>RTKIVVKVHMPCDKSRAKAVALAASVNGVDVVEITGEDKDRLEVVGRGIDPVRLVALLRE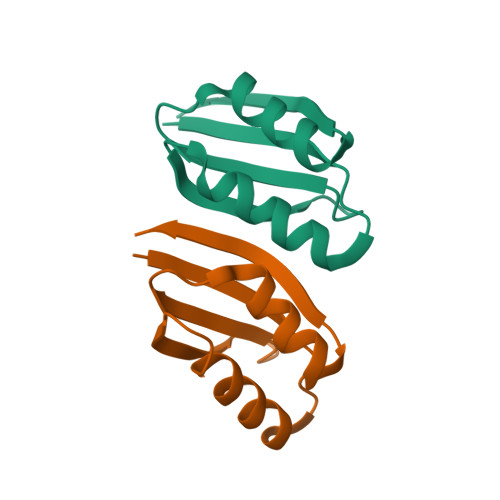KCGLAELLMVELV[2x]> TLT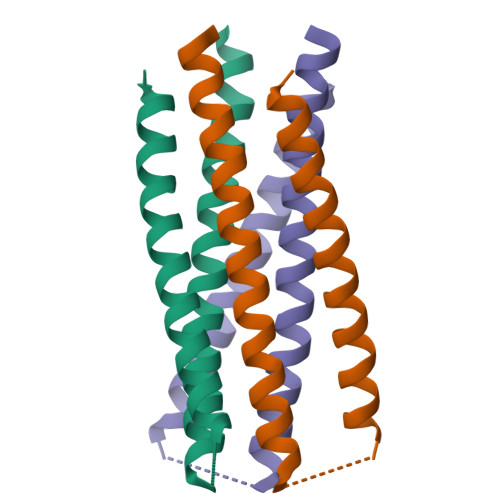VQARQLLSGIVQQQNDLLRAIEAQQHLLQLTVWGIKQLQARSGGRGGWMEWDREINNYTSLIHSLIEKSQNQQEKNEQELLEL4-cyano-~{N}-[2-(piperidin-1-ylmethyl)-1~{H}-benzimidazol-5-yl]benzamide 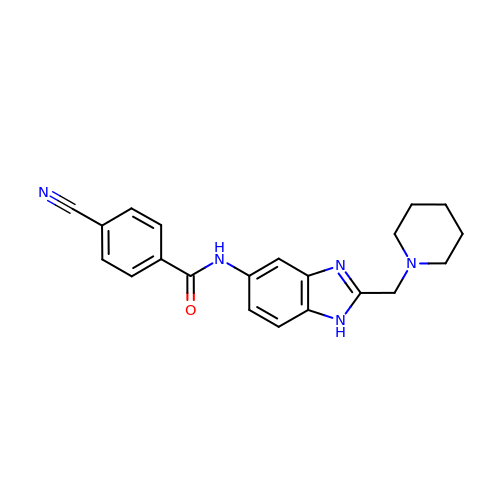| C21 H21 N5 O | PYUJNKLBJTZGDT-UHFFFAOYSA-N> GLGDELEEVIVEKTKQTVASISSGPKHTQKVPILTANETGATMPVLPSDSIETRTTYMHFNGSETDVECFLGRAACVHVTEIQNKDATGIDNHREAKLFNDWKINLSSLVQLRKKLELFTYVRFDSEYTILATASQPDSANYSSNLVVQAMYVPPGAPNPKEWDDYTWQSASNPSVFFKVGDTSRFSLPYVGLASAYNCFYDGYSHDDAETQYGITVLNHMGSMAFRIVNEHDEHKTLVKIRVYHRAKHVEAWIPRAPRALPYTSIGRTNYPKNTEPVIKKRKGDIKSY;> SPNVEACGYSDRVQQITLGNSTITTQEAANAVVCYAEWPEYLPDVDASDVNKTSKPDTSVCRFYTLDSKTWTTGSKGWCWKLPDALKDMGVFGQNMFFHSLGRSGYTVHVQCNATKFHSGCLLVVVIPEHQLASHEGGNVSVKYTFTHPGERGIDLSSANEVGGPVKDVLYNMNGTLLGNLLIFPHQFINLRTNNTATIVIPYINSVPIDSMTRHNNVSLMVIPIAPLTVPTGATPSLPITVTIAPMCTEFSGIRSKSIVPQ;> GLPTTTLPGSGQFLTTDDRQSPSALPNYEPTPRIHIPGKVHNLLEIIQVDTLIPMNNTHTKDEVNSYLIPLNANRQNEQVFGTNLFIGDGVFKTTLLGEIVQYYTHWSGSLRFSLMYTGPALSSAKLILAYTPPGARGPQDRREAMLGTHVVWDIGLQSTIVMTIPWTSGVQFRYTDPDTYTSAGFLSCWYQTSLILPPETTGQVYLLSFISACPDFKLRLMKDTQTISQTVALTE;> GAQVSTQKSGSHENQNILTNGSNQTFTVIN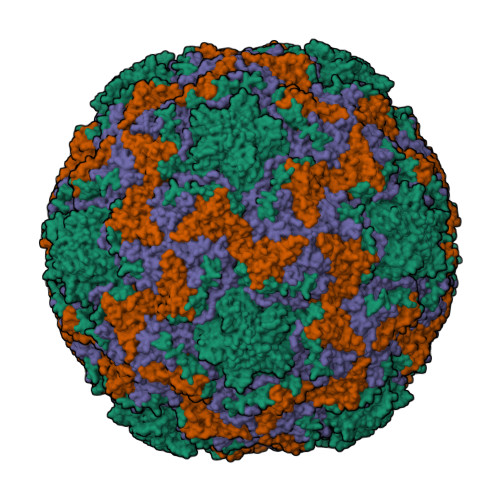YYKDAASTSSAGQSLSMDPSKFTEPVKDLMLKGAPALN> XVNAKQYHRILKRRQA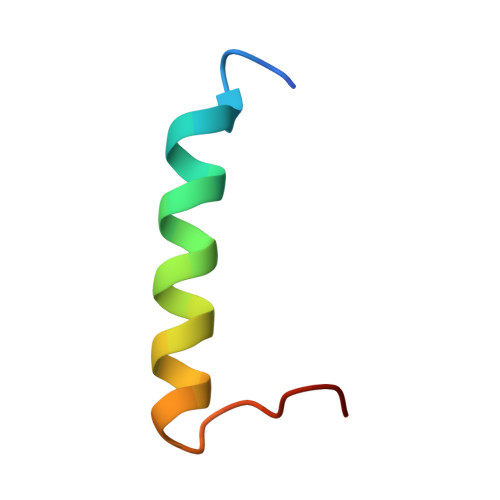RAKLEAEGKIPKERX>SNAMSNYKIPTLTIAGSDSSGGAGIQADLKTFSAIGTYGMSVITAITAQNTKGVFAVEDLNKKIIKKQIEAVFEDIPPRAVKIGMVSSPEIILEIVENLKKYNPKYLVVDPVMISKSGYYLLKPEAKENLIKYLIPLAYIITPNIPEAEEITGIKIHNVDDMKRVGEEILQLGPKFVLMKGGHLDGEAVDILVGKNIFKVYKSERIDKKNTHGTGCTLSSAITSYLALGYEITEAVNLSKIYITEAIKRSFDIGHGVGPVHHFY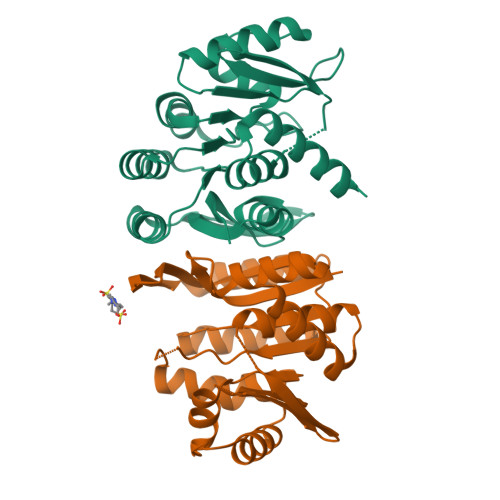KFE[2x]>MSDYGFANIEEAKADAIFKLNAQYHQDEDPKKVNMSVGAYRDDTGKPWILPAVKKASKIVEEQASFNHEYLPIAGLPRFTKAAAEVLFRPNPHLLSEDRVASMQSVSGTGANFLAASFIETFYVKHTGAHVYISNPTWPVHRTLWEKLGVTVETYPYWDAKNRSFDYEGMLSTIKSAPEGSIFLLHACAHNPTGIDPTREQWLSIFESLLSRKHLVVFDIAYQGFASGDLNRDSWALNEFVKYNKDFFVCQSFAKNMGLYGERTGCMHYVAKDASTKNKVLSQLCIVQRNTISNPPAYGARIAAEILNSPQLFAEWEQDLKTMSSRIIEMRKRLRDSLVALKTPGSWDHITQQIGMFSFTGLTPAQVQFCQERYHLYFSANGRISMAGLNNSNVEHVAQAFNHAVRELPLEHHHHHH[2x]

L-aspartate aminotransferase (AST, EC 2.6.1.1) is not only a key metabolic enzyme that links amino acid metabolism to carbohydrate metabolism through reversible transamination reaction but also an enzyme that regulates the cellular level of amino acid by catalyzing amino acid degradation and biosynthesis. AST generally forms a homodimer consisting of two active sites in the vicinity of subunit interfaces; these active sites bind to its cofactor PLP and substrate independently. Each subunit is composed of three parts: large domain, small domain, and N-terminal arm. The active site is situated in the cavity formed by two large domains and one small domain.

In this study, to suggest a broader view of the three-dimensional structure and show the structural features of PLP-family proteins, we determined the crystal structure of AST from Schizosaccharomyces pombe. The structure of SpAST forms a very stable homodimer with an unusually extended interface. Each subunit of SpAST folds up into three spatially and functionally distinct regions: a large domain, a small domain, and the N-terminal arm. Two tyrosine residues in both of the large domains, Tyr298 in helix α11, forms a face-to-face pi interaction with each other within a distance of 4 Å, contributing to stable dimerization of the dimer. Unexpectedly, two additional electron densities were found at the active site and the surface that could be fitted to phosphate and glycerol molecules. A clear density that could be fitted in most likely a phosphate was found in the active site of SpAST. Interestingly, the phosphate was located in the corresponding position of the phosphate moiety of PLP. The phosphate moiety interacts with the main chain of Gly108 and Thr109 and the side chain of Arg263 and Tyr70. Notably, the electron densities of Arg289 and Lys255 in SpAST were somewhat poor, but unambiguously, the positions of Arg289 and Lys255 side chains were located away from the cofactor or inhibitor from SpAST. This was presumably owing to the absence of its substrate or inhibitor.ethyl (2,3,4-trimethoxy-6-octanoylphenyl)acetate | C21 H32 O6 | 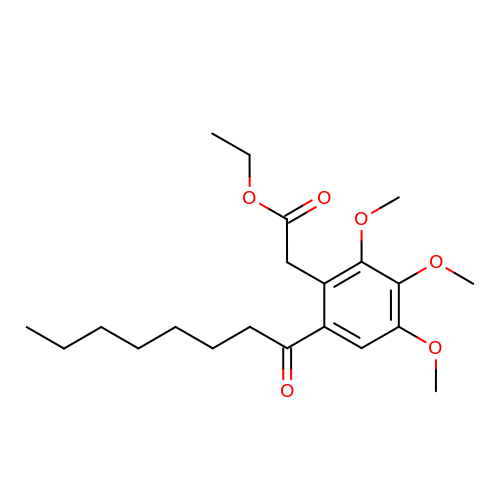WCYMJQXRLIDSAQ-UHFFFAOYSA-N>[6x]MERLDIFGVPIDRVTMIQAVDILNNFLQENRLHIVATPNAEIVMMAQKDKEYMEILNNTDLNVPDGSGIVFASKVFKKPLPERVAGFDLMLEFIKGISSKGVKIYLLGAACQVAEQARANLEKLYPGVKIVGTHHGYFTEEEENKIIEEINNKGAEVLFVALGAPKQEKWIYKNKDKLKVKIAMGVGGSFDVIAG

The TagA N-acetylmannosamine transferase catalyzes the first committed step in WTA biosynthesis. The TagA glycosyltransferase (GT) then appends ManNAc from a UDP-ManNAc donor, producing a C55-PP-GlcNAc-ManNAc disaccharide-lipid product (lipid-β). To gain insight into the mechanism of catalysis, we determined the 2.0 Å crystal structure of the TagA enzyme from Thermoanaerobacter italicus (TagAΔC, residues Met1-Gly195). TagAΔC contains the highly conserved amino acid region that defines the WecB/TagA/CpsF family, but lacks 49 C-terminal residues that target the protein to the membrane (see below).

To define the enzyme active site, we determined the structure of the SeMet-labeled TagAΔC:UDP complex at 3.1 Å resolution. The crystal structure visualizes the enzyme-product complex, as steady-state kinetics studies of B. subtilis TagA have shown that the enzyme operates via an ordered Bi-Bi mechanism in which UDP-ManNAc binds first and UDP is released last. The complex crystallizes as a dimer of trimers in the P21 space group, with six molecules in each asymmetric unit. The coordinates of the apo- and UDP-bound forms of TagAΔC are nearly identical (RMSD of 0.18 Å), suggesting that the enzyme binds UDP through a lock-and-key mechanism. In each protomer, UDP contacts the β7-H8 motif within the Rossmann-like fold, as well as the C-terminal edge of strand β5. The uracil base is engaged in pi stacking with Tyr137 (β6-H7 loop), while Asp191 (H9) contacts the ribose sugar. However, the C2 hydroxyl group in each UDP molecule forms a hydrogen bond with the backbone carbonyl of Val192 (H9) located in the adjacent subunit, which may explain why the complex crystallized as a trimer. The trimeric oligomer observed in the structure of the complex is presumably an artifact of crystallization, as AUC experiments using the native TagAΔC performed in the presence of saturating amounts of UDP indicate that similar to apo-TagAΔC, the UDP-bound protein fits best to a monomer-dimer equilibrium model rather than monomer-trimer or dimer-trimer equilibrium models (Kd = 3.5 ± 0.4 μM in the presence of 10:1 UDP:TagA). Interestingly, in the crystal structure of the TagAΔC:UDP complex, the β-phosphate group of UDP extends inward toward the pocket. As UDP is a competitive inhibitor of the UDP-ManNAc substrate, it is likely that these ligands bind to the same site on the enzyme, such that the ManNAc moiety within UDP-ManNAc is projected into the pocket where it can interact with the conserved side chains of residues Thr37, Gln167 or Glu168.>MATEQIQHIAIVGCVH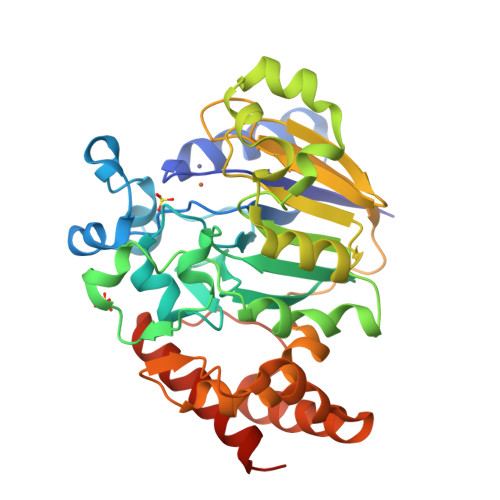GKYREMYRQLSEYEKSTGKEISFVICTGDMQTLRYEADLVYLKVPPKYKQMGDFHLYYEGKEKAPYLTLFIGGNAESSNVLLHLYNGGFVCFNMYYLGVCSCININGLRIVGVSGIYKSFDEKKPYTYPPSPNDVVSLFHTRNYVIQMLSNLSQSSQIDISLSHDWPQGIVMKGNYKQLYRFQPGFKKDGASLGSPINKVILNTLKPKYWISGHMHCEYHAEEGPTHFIALGKIGYKNAISYLDLPLKQKTDLEYDKDWVCNLIMTWPAFSNKAQFPDLSYSISELLSKRTKELDKKIIELWEKYIGLKIIYDSDTFDIQFTSRRFYIEKIYNELNINHHHHHH[5x]> MSGHHHHHHVILEANKIRKSYGNKLNKQEVLKGIDIHIEKGEFVSIMGASGSGKTTLLNVLSSIDQVSHGTIHINGNDMTAMKEKQLAEFRKQHLGFIFQDYNLLDTLTVKENILLPLSITKLSKKEANRKFEEVAKELGIYELRDKYPNEISGGQKQRTSAGRAFIHDPSIIFADEPTGALDSKSASDLLNKLSQLNQKRNATIIMVTHDPVAASYCGRVIFIKDG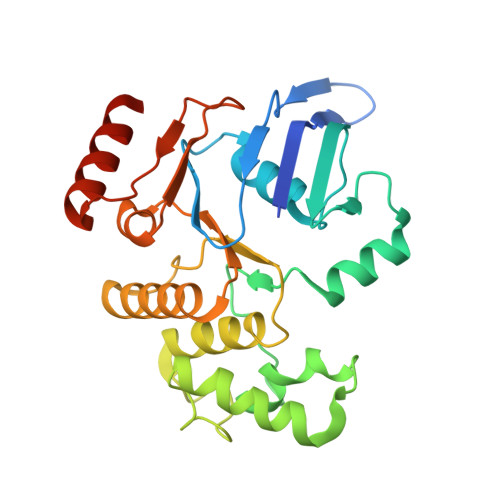QMYTQLNKGGQDRQTFFQDIMKTQGVLGGVQHEH> MGSSHHHHHHSHGSMEVLKNIRIYPLSNFITSTKNYINLPNELRNLISEEQESKLGFLHIIESDFKPSVALQKLVNCTTGDEKILIIDIVSIWSQQKQRQHGAIYMNSLSCI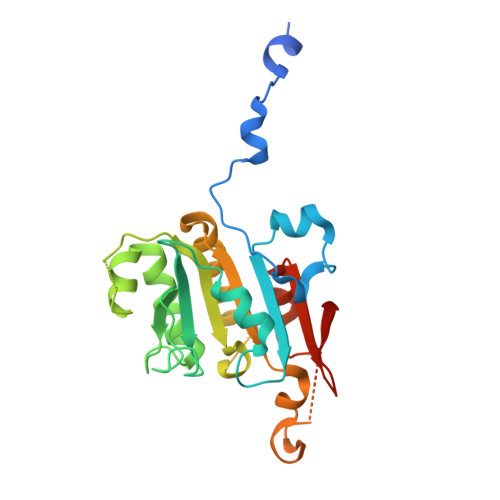NITGLIVFLELLYDSPMDALRRCQVDNFNFQLRGIVIDNLSFLNFESDKNYDVINLSKFEKLFKILRKLREFLGCWIITKSFPTDFYNGIENTLVDKWSIKRKSGVTLYPTKLPDSYMKGMDLIIYREVVDGRPQYRRIAALEE>LHLDQTPSRQPIPSEGLQLHLPQVLADAVSRLVLGKFGDLTDNFSSPHARRKVLAGVVMTTGTDVKDAKVISVSTGTKCINGEYMSDRGLALNDCHAEIISRRSLLRFLYTQLELYLNNKDDQKRSIFQKSERGGFRLKENVQFHLYISTSPCGDARIFSPHEPILEEPADRHPNRKARGQLRTKIESGEGTIPVRSNASIQTWDGVLQGERLLTMSCSDKIARWNVVGIQGSLLSIFVEPIYFSSIILGSLYHGDHLSRAMYQRISNIEDLPPLYTLNKPLLSGISNAEARQPGKAPNFSVNWTVGDSAIEVINATTGKDELGRASRLCKHALYCRWMRVHGKVPSHLLRSKITKPNVYHESKLAAKE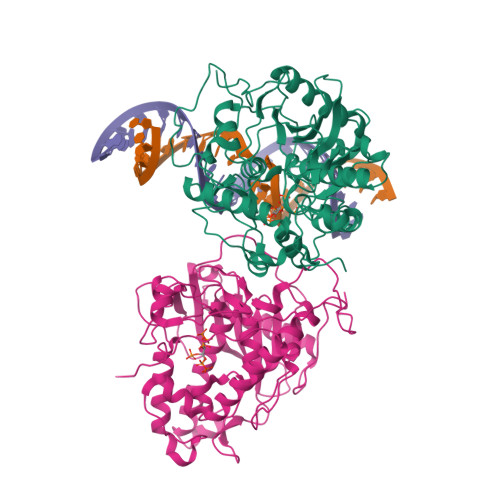YQAAKARLFTAFIKAGLGAWVEKPTEQDQFSLTP[2x]>[4x]M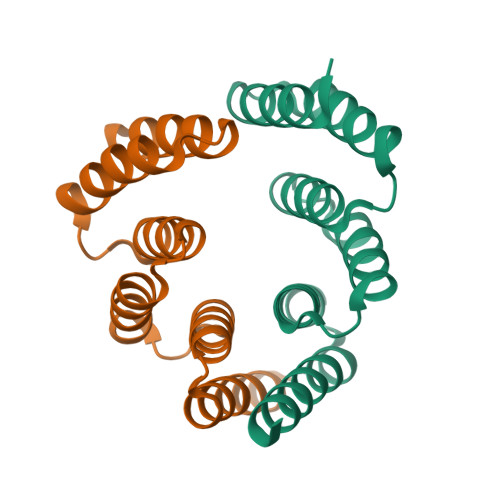GNSIKTLSNLANLLAQEGKAEEAIKYMRKAVSLDPNNIKTLSNLANLLAQEGKAEEAIKYMRKAVSLDPNNIKTLSNLAVLLAQEGKAEEAIKYMRKAVSLIDKAAKG> MKKGSANEDMPVERI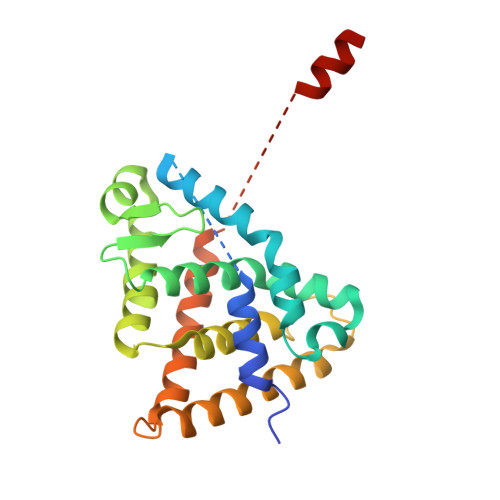LEAELAVEPKTETYVEANMGLNPSSPNDPVTNICQAADKQLFTLVEWAKRIPHFSELPLDDQVILLRAGWNELLIASFSHRSIAVKDGILLATGLHVHRNSAHSAGVGAIFDRVLTELVSKMRDMQMDKTELGCLRAIVLFNPDSKGLSNPAEVEALREKVYASLEAYCKHKYPEQPGRFAKLLLRLPALRSIGLKCLEHLFFFKLIGDTPIDTFLMEMLEAPHQMT>[2x]MSSSKTIRSRSIWDDAHAMLEKAKAEGISTVWDRAAEQTPACKFGELGTCCRNCIMGPCRIANRKDGKMRLGVCGADADVIVARNFGRFIAGGAAGHSDHGRDLIETLEAVAEGKAPGYTIRDVAKLRRIAAELGVADAATRPAHDVAADLVTICYNDFGSRRNALAFLARAPQVRRDLWQRLGMTPRGVDREIAEMMHRTHMGCDNDHTSLLVHAARTALADGWGGSMIGTELSDILFGTPRPRQSTVNLGVLRKDAVNILVHGHNPVVSEMILAATREPAVRQAAQDAGAADINVAGLCCTGNELLMRQGIPMAGNHLMTELAIVTGAADAIVADYQCIMPSLVQIAACYHTRFVTT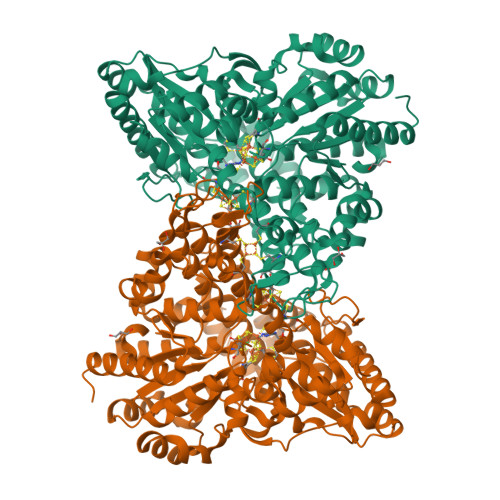SPKGRFTGATHVEVHPHNAQERCREIVMLAIDAYTRRDPARVDIPSQPVSIMSGFSNEAILEALGGTPKPLIDAVVAGQIRGFVGIVGCNNPKIRQDSANVTLTRELIRRDIMVLATGCVTTAAGKAGLLVPEAASKAGEGLAAVCRSLGVPPVLHMGSCVDNSRILQLCALLATTLGVDISDLPVGASSPEWYSEKAAAIAMYAVASGIPTHLGLPPNILGSENVTAMALHGLQDVVGAAFMVEPDPVKAADMLEAHIVARRARLGLTS> MGKTNDWLDFDQLAEEKVRDALKPPSM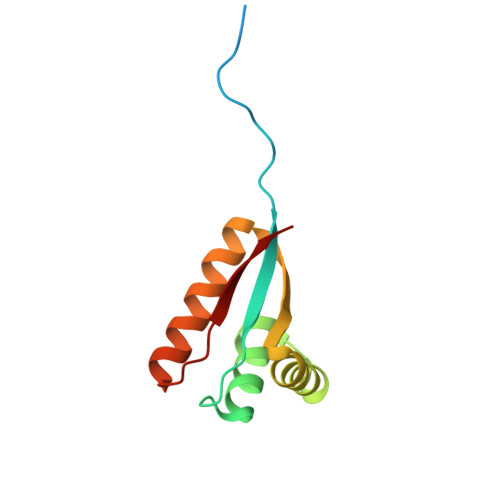YKVILVNDDYTPMEFVIDVLQKFFSYDVERATQLMLAVAYQGKAICGVFTAEVAETKVAMVNKYARENEHPLLCTLEKA> MVEATAQETDRPRFSFSIAAREGKARTGTIEMKRGVIRTPAFMPVGTAATVKALKPETVRATGADIILGNTYHLMLRPGAERIAKLGGLHSFMGWDRPILTDSGGYQVMSLSSLTKQSEEGVTFKSHLDGSRHMLSPERSIEIQHLLGSDIVMAFDECTPYPATPSRAASSMERSMRWAKRSRDAFDSRKEQAENAALFGIQQGSVFENLRQQSADALAEIGFDGYAVGGLA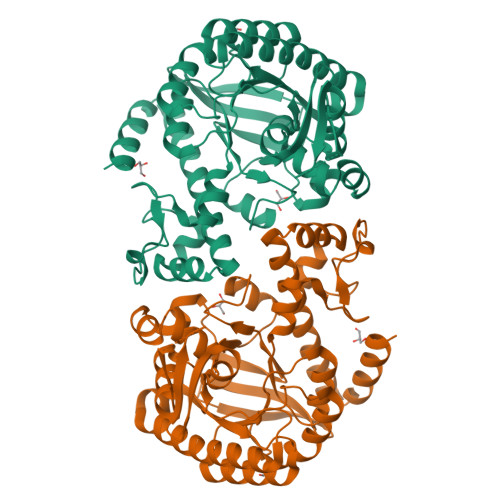VGQGQDEMFRVLDFSVPMLPDDKPHYLMGVGKPDDIVGAVERGIDMFDCVLPTRSGRNGQAFTWDGPINIRNARFSEDLKPLDSECHCAVCQKWSRAYIHHLIRAGEILGAMLMTEHNIAFYQQLMQKIRDSISEGRFSQFAQDFRARYFARNS> MDLSNMESVVESALTGQRTKIVVKVHMPCGKSRAKAMALAASVNGVDSVEITGEDKDRLVVVGRGIDPVRLVAL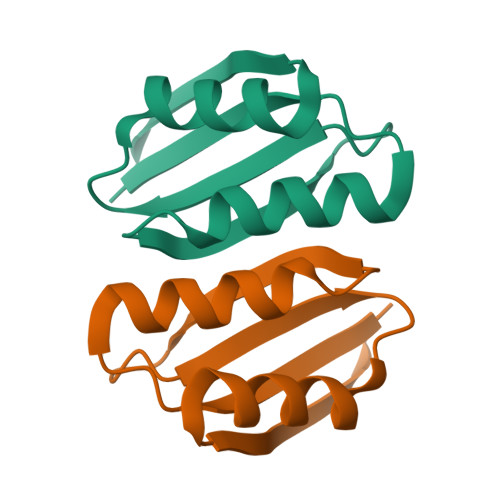LREKCGLAELLMVELVEKEKTQLAGGKKGAYKKHPTYNLSPFDYVEYPPSAPIMQDINPCSTM> MGEALKILNNIRTLRAQARECTLETLEEMLEKLEVVVNER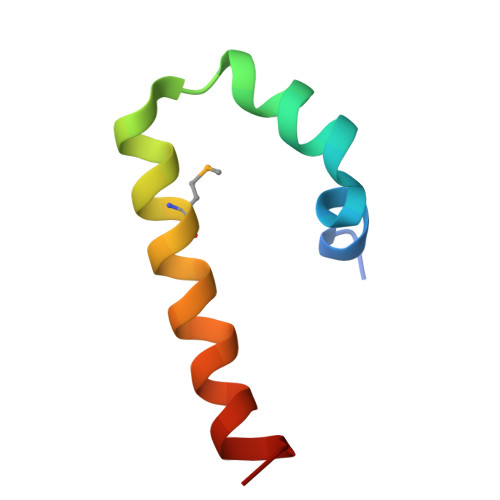REEESA> MLRRALEEAIAQALKEMGVPVRLKVARAPKDKPGDYGVPLFALAKELRKPPQAIAQELKDRLPLPEFVEEAVPVGGYLNFRLRTEALLREALRPKAPFPRRPGVVLVEHTSVNPNKELHVGHLRNIALGDAIARILAYAGREVLVLNYIDDTGRQAAETLFALRHYGLTWDGKEKYDHFAGRAYVRLHQDPEYERLQPAIEEVLHALERGELREEVNRILLAQMATMHALNARYDLLVWESDIVRAGLLQKALALLEQSPHVFRPREGKYAGALVMDASPVIPGLEDPFFVLLRSNGTATYYAKDIAFQFWKMGILEGLRFRPYENPYYPGLRTSAPEGEAYTPKAEETINVVDVRQSHPQALVRAALALAGYPALAEKAHHLAYETVLLEGRQMSGRKGLAVSVDEVLEEATRRARAIVEEKNPDHPDKEEAARMVALGAIRFSMVKTEPKKQIDFRYQEALSFEGDTGPYVQYAHARAHSILRKAGEWGAPDLSQATPYERALALDLLDFEEAVLEAAEERTPHVLAQYLLDLAASWNAYYNARENGQPATPVLTAPEGLRELRLSLVQSLQRTLATGLDLLGIP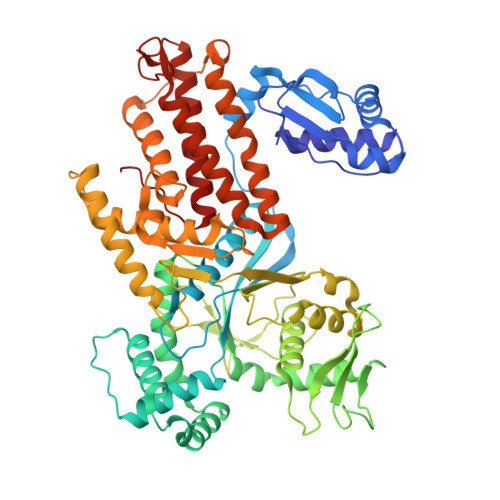APEVM3-{5-[(6-amino-1H-pyrazolo[3,4-b]pyridin-3-yl)methoxy]-2-chlorophenoxy}-5-chlorobenzonitrile | C20 H13 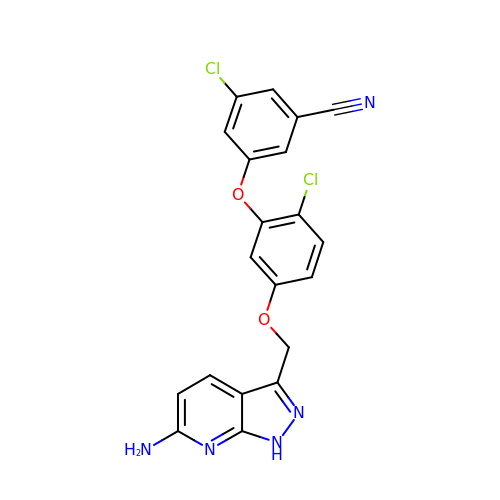Cl2 N5 O2 | KXDIHAQCVNNLIB-UHFFFAOYSA-N>[4x]RVLQVDIVPSQGEISVGESKFFLCQVAGDAKDKDISWFSPNGEKLSPNQQRISVVWNDDDSSTLTIYNANIDDAGIYKCVVTAEDGTQSEATVNVKIFQKLMFKNAPTPQEF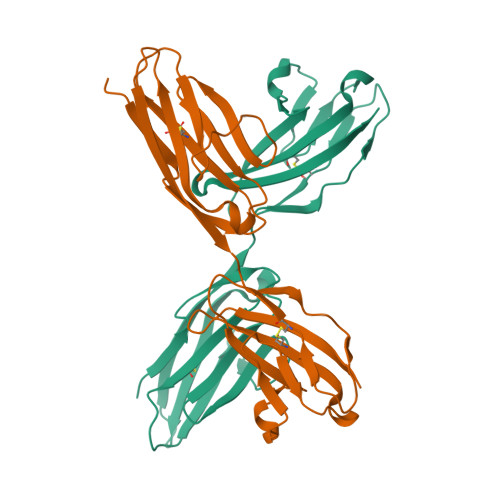KEGEDAVIVCDVVSSLPPTIIWKHKGRDVILKKDVRFIVLSNNYLQIRGIKKTDEGTYRCEGRILARGEINFKDIQVIV>QYLLPEAKAQDSDKICVVINLDETLVHSSFKPVNNADFIIPVEIDGVVHQVYVLKRPHVDEFLQRMGELFECVLFTASLAKYADPVADLLDKWGAFRARLFRESCVFHRGNYVKDLSRLGRDLRRVLILDNSPASYVFHPDNAVPVASWFDNMSDTELHDLLPFFEQLSRVDDVYSVLRQ[2x];>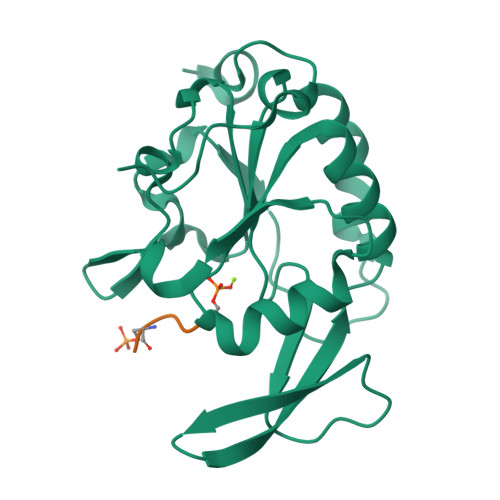EDLSPPSPPLPK[2x]> MGHHHHHHMPEINTNHLDKQQVQLL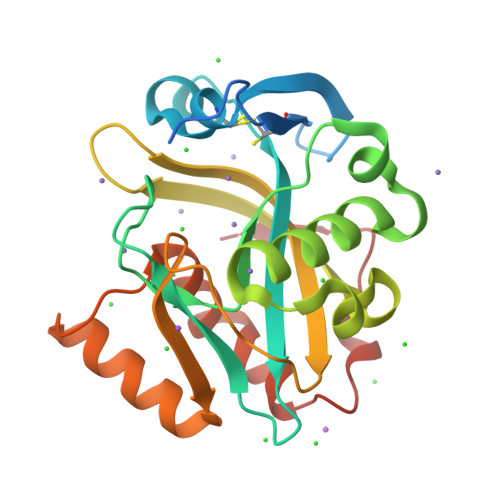AEMCILIDENDNKIGAETKKNCHLNENIEKGLLHRAFSVFLFNTENKLLLQQRSDAKITFPGCFTNTCCSHPLSNPAELEESDALGVRRAAQRRLKAELGIPLEEVPPEEINYLTRIHYKAQSDGIWGEHEIDYILLVRMNVTLNPDPNEIKSYCYVSKEELKELLKKAASGEIKITPWFKIIAATFLFKWWDNLNHLNQFVDHEKIYRM S-[2-(propanoylamino)ethyl] (2S)-2-[(8S,9S,10R,13S,14S,17R)-10,13-dimethyl-3-oxo-6,7,8,9,10,11,12,13,14,15,16,17-dodecahydro-3H-cyclopenta[a]phenanthren-17-yl]propanethioate (non-preferred name) | C27 H39 N O3 S | 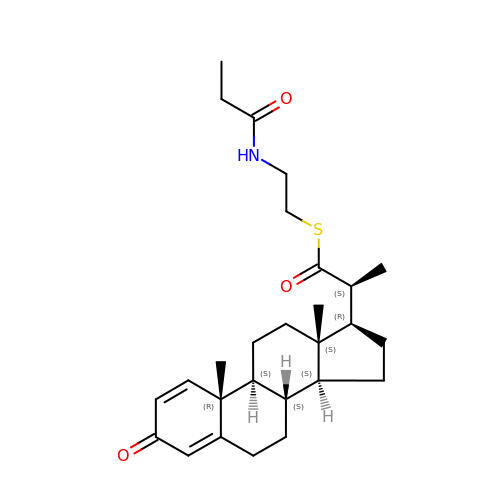NPTBAEOEUMZYQL-CTKPXJAYSA-N> MEDLCVANTLFALNLFKHLAKASPTQNLFLSPWSISSTMAMVYMGSRGSTEDQMASVLQFNEVGAAADKIHSSFRSLSSAINASTGNYLLESVNKLFGEKSASFREEYIRLCQKYYSSEPQAVDFLECAEEARKKINSWVKTQTKGKIPNLLPEGSVDGDTRMVLVNAVYFKGKWKTPFEKKLNGLFPFRVNSAQRTPVQMMYLREKLNIGYIEDLKAQILELPYAGDVSMFLLLPDEIADVSTGLELLESEITYDKLNKWTSKDKMAEDEVEVY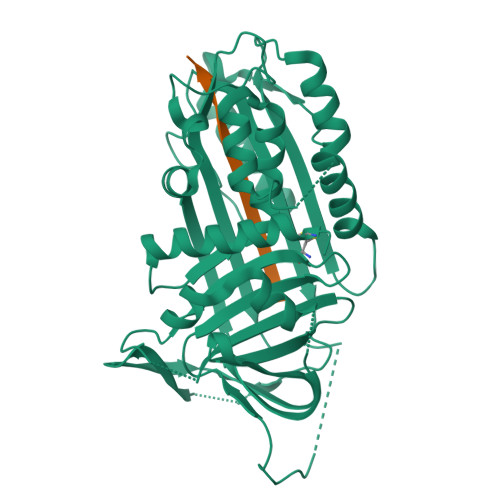IPQFKLEEHYELRSILRSMGMEDAFNKGRANFSGMSERNDLFLSEVFHQAMVDVNEEGTEAAAGTGGVMTGRTGHGGPQFVADHPFLFLIMHKITNCILFFGRFSSP;> XTEAAAGMGGVMTGR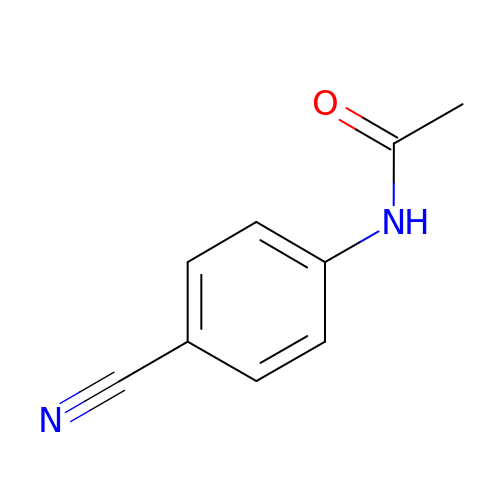~{N}-(4-cyanophenyl)ethanamide | C9 H8 N2 O | UFKRTEWFEYWIHD-UHFFFAOYSA-N>GHMSWSPSLTTQTCGAWEMKERLGTGGFGNVIRWHNQETGEQIAIKQCRQELSPRNRERWCLEIQIMRRLTHPNVVAARDVPEGMQNLAPNDLPLLAMEYCQGGDLRKYLNQFENCCGLREGAILTLLSDIASALRYLHENRIIHRDLKPENIVLQQGEQRLIHKIIDLGYAKELDQGELCTEFVGTLQYLAPELLEQQKYTVTVDYWSFGTLAFECITGFRPFLPNWQPVQWHSKVRQKSEVDIVVSEDLNGTVKFSSSLPYPNNLNSVLAERLEKWLQLMLMWHPRQRGTDPTYGPNGCFKALDDILNLKLVHILNMVTGTIHTYPVTEDESLQSLKARIQQDTGIPEEDQELLQEAGLALIPDKPATQCISDGKLNEGHTLDMDLVFLFDNSKITYETQISPRPQPESVSCILQEPKRNLAFFQLRKVWGQVWHSIQTLKEDCNRLQQGQRAAMMNLLRNNSCLSKMKNSMASMSQQLKAKLDFFKTSIQIDLEKYSEQTEFGITSDKLLLAWREMEQAVELCGRENEVKLLVERMMALQTDIVDLQRSPMGRKQ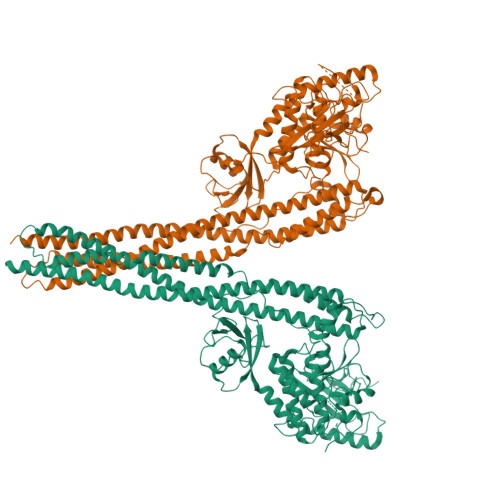GGTLDDLEEQARELYRRLREKPRDQRTEGDSQEMVRLLLQAIQSFEKKVRVIYTQLSKTVVCKQKALELLPKVEEVVSLMNEDEKTVVRLQEKRQKELWNLLKIACSKVRGPV[5x]>MHHHHHHMITVDKRPSSRGYDDWRLSDIPQYKDGISTYEFVRATHEADYRTHQAEPVAGRTFGFNGIGRLTEVALHMPTRYTLHDQSSQYKESPSFFQGLMGVPDRGPVDLAAFQRETEELATAFENNGIKVHWVDYPEEPANPYGPLMGHVFLSWGSIWRGGSVISRFGFLPGMVGVSEYLAKWAWNTLNIPPLVAITEGAMEPGACNMIADEVLVTCLSASYDQRGTDQLVAAISKTSGTEEFHNLQLRPAVEGFFNKATGACAHPDININAIDVGKLVVSPAALDWDARTWLYDNNFELIEADPDEQREFLAPCNVLLLEPGKVIAHADCHKTNQKIRDAGVEVIEVTGTEIRKACGGIKCRVMQINREPGPTLADVRNRVWR[6x]

Mycobacterium sp. JS330 produces 2-nitroimidazole nitrohydrolase (NnhA) that circumvents 2NI activation, conferring 2NI resistance by hydrolysing it to nitrite and imidazol-2-one (IM2O) instead. The initial characterization of NnhA indicated that, unlike most other known enzymes that degrade nitroaromatic compounds, NnhA is a hydrolase that functions without catalytic metal ions, molecular oxygen, or other cofactors. Despite low sequence similarity and limited occurrence in a few soil-dwelling mycobacteria and Actinomycetota, NnhA maintains the α/β propeller fold characteristic of GME superfamily enzymes and forms an unusual hexameric ring structure formed by a trimer of domain-swapped dimers. The residues in the active site of NnhA appear somewhat conserved in comparison to the ADI and DDAH, with the catalytic histidine, glutamic acid, and cysteine residues present in NnhA as H260, E197, and C357.

Using this process, we identified a variant of NnhA containing three amino acid substitutions (T2I, G14D, and K73R) that exhibited a substantial increase in soluble protein production in E. coli compared to the WT when analyzed on an SDS-PAGE gel. We isolated and purified this variant protein (referred to as “soluble NnhA”) with a yield of 8 mg of protein per liter of E. coli culture and compared its catalytic activity with the WT protein. With data close to 2 Å resolution (2.04 and 2.16 Å), the quality of the electron density maps was good and showed unambiguous density from residue R11 to R379 at the C-terminus. In the unit cell of the P1 space group obtained for soluble NnhA, three homodimers are arranged to create a hexameric ring, with a large pore in the middle. There are three dimers found in the hexameric structure, and therefore each protomer has interactions with three other protomers, including its dimerization partner. NnhA also has an N-terminal extension that makes extensive interactions with the adjoining protomer to form a domain-swapped homodimer, the presence of which also distorts the first β-sheet in the proceeding ββαβ motif. The third T2I mutation is not resolved in the structure as it is located at the start of the polypeptide near the N-terminal His-tag. Both G14D and K73R introduce oppositely charged residues that are located such that they could potentially introduce a salt-bridge interaction to strengthen the dimer interface. However, the minimum distance observed between them in all the crystal structures was 6.2 Å, which is further than the expected 2–4 Å for a salt bridge but may still be relevant when the protein is in solution and in a dynamic state. The conformational flexibility within the oligomerized complex was also supported by the crystal structure, where high B-factors were observed in surface residues of some protomers but not others.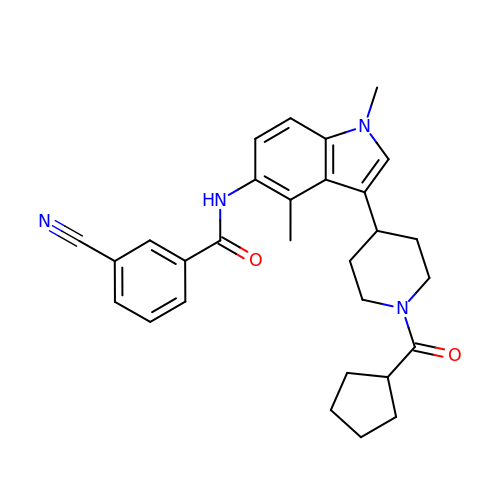3-cyano-N-{3-[1-(cyclopentanecarbonyl)piperidin-4-yl]-1,4-dimethyl-1H-indol-5-yl}benzamide | C29 H32 N4 O2 | HQKLWNNRWVVUSC-UHFFFAOYSA-N4-[2-(1,1,3,3-tetramethyl-2,3-dihydro-1H-1,3-benzodisilol-5-yl)-1,3-dioxolan-2-yl]benzoic 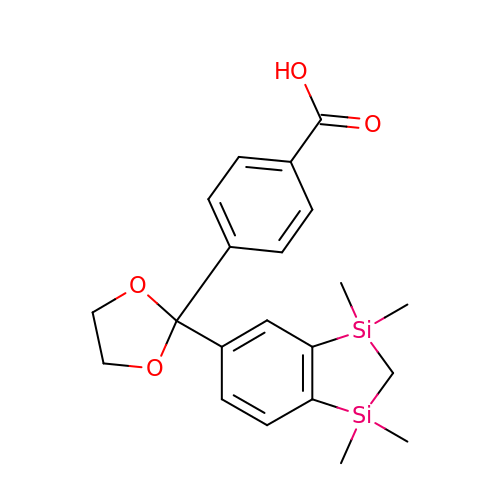acid | C21 H26 O4 Si2 | JJYIDLOYXKNNAS-UHFFFAOYSA-N>[2x]MNPTIIRARAPLRLGLAGGGTDVAPYADTFGGYVLNATIDRYAYAVIKTLTIPAVRFVSTDQQVEKHQLISEPLELNGTLNLHKAVYNHMIRNYNHGKPIALELSTFCDAPAGSGLGSSSTLVVVMIKAFVELLNLPLDDYAIAQLAYRIERVDCGLAGGRQDQYSATFGGFNFMEFYEEERTIVNPLRIKNWVLCELEASLVLFYTGVSRESAKIIQDQSDNVVSHKTAAIEAMHGIKREALVMKEALLKGDFKAFVASMRLGWDNKKNSARTVSNAHIDEIYDAAIRAGAQAGKVSGAGGGGFMLFFVPTEKRMDLIRTLGEYDGQVSNCHFTKNGTQAWRIAN

Here, we present the structure of WcbL from Burkholderia pseudomallei. A critical step in the synthesis of heptoses is their 1-O phosphorylation, mediated by kinases such as HldE or WcbL. We report that WcbL operates through a sequential ordered Bi-Bi mechanism, loading the heptose first and then ATP. The protein forms a head-to-tail dimer, with the two active sites facing away from the dimer interface, in line with the native molecular weight predicted from size-exclusion chromatography.

Furthermore, soaking of native crystals with glycerol or mannose showed that these two sugars both bind in the sugar-phosphate binding pocket, where the sugar is expected. The glycerol and mannose complex crystals had a higher proportion of the monoclinic cell: these data could be processed, and the models refined well in both space groups. However, ligand electron density was significantly better in the orthorhombic space group for both of these complexes, and therefore all structures were refined in the orthorhombic cell.> MSMSTSTEVIAHHWAFAIFLIVAIGLCCLMLVGGWFLGGRARARSKNVPFESGIDSVGSARLRLSAKFYLVAMFFVIFDVEALYLFAWSTSIRESGWVGFVEAAIFIFVLLAGLVYLVRIGALDWTPARSRRERMNPETNSIANRQR;> MSWISPELIEILLTILKAVVILLVVVTCGAFMSFGERRLLGLFQNRYGPNRVGWGGSLQLVADMIKMFFKEDWIPKFSDRVIFTLAPMIAFTSLLLAFAIVPVSPGWVVADLNIGILFFLMMAGLAVYAVLFAGWSSNNKYSLLGAMRASAQTLSYEVFLGLSLMGVVAQAGSFNMTDIVNSQAHVWNVIPQFFGFITFAIAGVAVCHRHPFDQPEAEQELADGYHIEYSGMKFGLFFVGEYIGIVTISALMVTLFFGGWQGPLLPPFIWFALKTAFFMMMFILIRASLPRPRYDQVMSFGWKICLPLTLINLLVTAAVILWQAQ;> MEFAFYICGLIAILATLRVITHTNPVHALLYLIISLLAISGVFFSLGAYFAGALEIIVYAGAIMVLFVFVVMMLNLGGSEIEQERQWLKPQVWIGPAILSAIMLVVIVYAILGVNDQGIDGTPISAKAVGITLFGPYVLAVELASMLLLAGLVVAFHVGREERAGEVLSNRKDDSAKRKTEEHA;> MIPLQHGLILAAILFVLGLTGLVIRRNLLFMLIGLEIMINASALAFVVAGSYWGQTDGQVMYILAISLAAAEASIGLALLLQLHRRRQNLNIDSVSEMRG;> MNMLALTIILPLIGFVLLAFSRGRWSENVSAIVGVGSVGLAALVTAFIGVDFFANGEQTYSQPLWTWMSVGDFNIGFNLVLDGLSLTMLSVVTGVGFLIHMYASWYMRGEEGYSRFFAYTNLFIASMVVLVLADNLLLMYLGWEGVGLCSYLLIGFYYTDPKNGAAAMKAFVVTRVGDVFLAFALFILYNELGTLNFREMVELAPAHFADGNNMLMWATLMLLGGAVGKSAQLPLQTWLADAMAGPTPVSALIHAATMVTAGVYLIARTHGLFLMTPEVLHLVGIVGAVTLLLAGFAALVQTDIKRVLAYSTMSQIGYMFLALGVQAWDAAIFHLMTHAFFKALLFLASGSVILACHHEQNIFKMGGLRKSIPLVYLCFLVGGAALSALPLVTAGFFSKDEILAGAMANGHINLMVAGLVGAFMTSLYTFRMIFIVFHGKEQIHAHAVKGVTHSLPLIVLLILSTFVGALIVPPLQGVLPQTTELAHGSMLTLEITSGVVAVVGILLAAWLWLGKRTLVTSIANSAPGRLLSTWWYNAWGFDWLYDKVFVKPFLGIAWLLKRDPLNSMMNIPAVLSRFAGKGLLLSENGYLRWYVASMSIGAVVVLALLMVLR;> MLLPWLILIPFIGGFLCWQTERFGVKVPRWIALITMGLTLALSLQLWLQGGYSLTQSAGIPQWQSEFDMPWIPRFGISIHLAIDGLSLLMVVLTGLLGVLAVLCSWKEIEKYQGFFHLNLMWILGGVIGVFLAIDMFLFFFFWEMMLVPMYFLIALWGHKASDGKTRITAATKFFIYTQASGLVMLIAILALVFVHYNATGVWTFNYEELLNTPMSSGVEYLLMLGFFIAFAVKMPVVPLHGWLPDAHSQAPTAGSVDLAGILLKTAAYGLLRFSLPLFPNASAEFAPIAMWLGVIGIFYGAWMAFAQTDIKRLIAYTSVSHMGFVLIAIYTGSQLAYQGAVIQMIAHGLSAAGLFILCGQLYERIHTRDMRMMGGLWSKMKWLPALSLFFAVATLGMPGTGNFVGEFMILFGSFQVVPVITVISTFGLVFASVYSLAMLHRAYFGKAKSQIASQELPGMSLRELFMILLLVVLLVLLGFYPQPILDTSHSAIGNIQQWFVNSVTTTRP;> MTITPQNLIALLPLLIVGLTVVVVMLSIAWRRNHFLNATLSVIGLNAALVSLWFVGQAGAMDVTPLMRVDGFAMLYTGLVLLASLATCTFAYPWLEGYNDNKDEFYLLVLIAALGGILLANANHLASLFLGIELISLPLFGLVGYAFRQKRSLEASIKYTILSAAASSFLLFGMALVYAQSGDLSFVALGKNLGDGMLNEPLLLAGFGLMIVGLGFKLSLVPFHLWTPDVYQGAPAPVSTFLATASKIAIFGVVMRLFLYAPVGDSEAIRVVLAIIAFASIIFGNLMALSQTNIKRLLGYSSISHLGYLLVALIALQTGEMSMEAVGVYLAGYLFSSLGAFGVVSLMSSPYRGPDADSLFSYRGLFWHRPILAAVMTVMMLSLAGIPMTLGFIGKFYVLAVGVQAHLWWLVGAVVVGSAIGLYYYLRVAV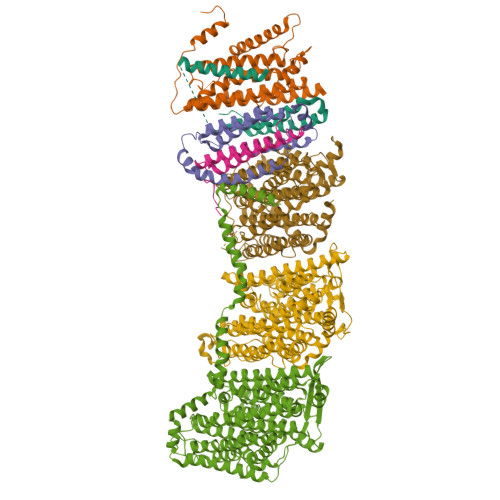SLYLHAPEQPGRDAPSNWQYSAGGIVVLISALLVLVLGVWPQPLISIVRLAMPLM>MAVIFHEKTKEFHIFNREVSYLMRIMENGQLENLYYGKVIRDKEDFGYLHEEAMRSQMSVCIPEPGILSMQYTRQEYPVYGTGDYRSPALTVLQENGSRLVDFSYVSHEIYKGKKGIPPLPSTYAESEDEAETLEVTLHDQVTDTDLVLTYTIYEDYPVITRNARFEQKGEQKIVLERAMSASVEFLDMDYELVQLSGAWSRERYVKNRKLEMGIQSVHSLNGTCGGAEHNPFIALKRPQTTENQGEVYGFSLVYSGNFLAQAEVSTFDMTRVMLGINPEDFSWELNQGESFQTPEVVMVYSDRGLNKMSQAYHRLYRTRLMRVTWRDKARPILLNNWEATYFDFNEEKILKIAEKAKEAGVELFVLDDGWFGARNDDYRGLGDWYVNLEKLPDGIAGLSRKVEALGLKFGLWVELEMVNKDSDLYRAHPDWLIGAPDRFESHARHQHVLDFSRKEVVDYIYKMIAKVLRESSISYIKWDMNRYMTEPYSRGADASQQGKVMHKYILGVYDLYTRLTTEFPEILFESCASGGARFDPAMLYFAPQTWTSDDTDASERTKIQYGTSYVYPVVSMGSHVSAVPNHQMHRMTPIETRANVAYFGTFGYELDLNLLSEAELESVKKQIAFMKEYRELIQVDGDFYRLLSPFEGNETAWMVVAQDKSRAVAAFYQRMNKVNASWIRFKLQGLDAGTLYEVS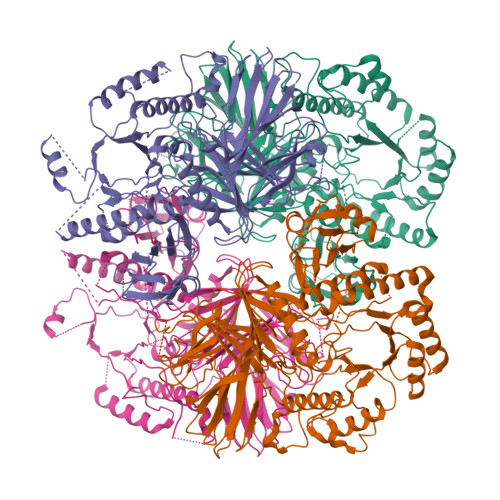CDMAPSASYDESLAKIYGIQTEENMVKTYRAYGDELMQVGIPIDREDLNKKGGDFASLLYTLKKVTD[4x]> PYASLTEIEHLVQSVCKSYRETCQLRLEDLLRQRSNIFSREEVTGYQRKSMWEMWERCAHHLTEAIQYVVEFAKRLSGFMELCQNDQIVLLKAGAMEVVLVRMCRAYNADNRT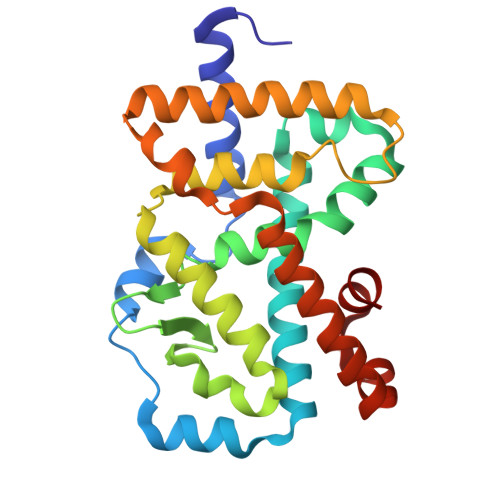VFFEGKYGGMELFRALGCSELISSIFDFSHSLSALHFSEDEIALYTALVLINAHRPGLQEKRKVEQLQYNLELAFHHHLCKTHRQSILAKLPPKGKLRSLCSQHVERLQIFQHLHPIVVQAAFPPLYKELFS>ETGTPMMPPVGVQASILSHDTIRITWADNSLPKHQKITDSRYYTVRWKTNIPANTKYKNANATTLSYLVTGLKPNTLYEFSVMVTKGRRSSTWSMTAHGATFELVPTSPPKDVTVVSKEGKPRTIIVNWQPPSEANGKITGYIIYYSTDVNAEIHDWVIEPVVGNRLTHQIQELTLDTPYYFKIQARNSKGMGPMSEAVQFRTPKADSSDKMPNDQALGSAGKGSRLPDLGSDYKPPMSGSNSPHGSPTSPLDSNGTKHHHHHH[2x];>[2x]ETGQPAQCRIQKCTTDFVSLTSHLNSAVDGFDSEFCKALRAYAGCTQRTSKACRGNLVYHSAVLGISDLMSQRNCSKDGPTSSTNPEVTHDPCNYHSHAGAREHRRGDQNPPSYLFCGLFGD;>[2x]PHLRTFKDNFQTCKVEGAWPLIDNNYLSVQVTNVPVVPGSSATATNKITIIFKAHHGCTDQKVYQAVTD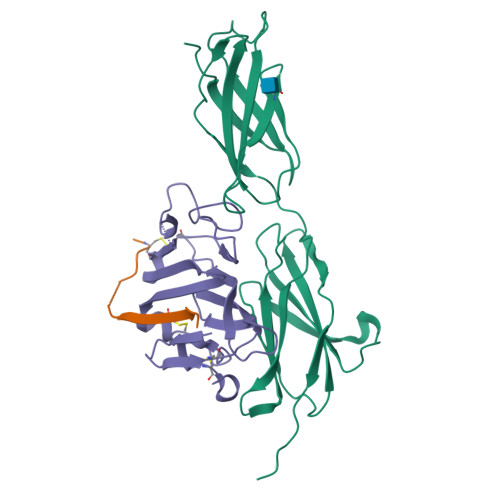DLPAAFVDGTTSGGDSDAKSLRIVERESGHYVEMHARYIGTTVFVRQVGRYLTLAIRMPEDLAMSYEESQDLQLCVNGCPLSERIDDGQGQVSAILGHSLPRTSLVQAWPGYTLETANTQCHEKMPVKDIYFQSCVFDLLTTGDANFTAAAHSALEDVEALHPRKERWHIFPSGTKHHHHHH> IERTAKQRLQALKANDEEAYLKLLDQAKDTRITHLLRQTDGFLKQLASSVRAQQRQAAERYGEQIDIPPDESDIDEDDEESGRKIDYYAVAHRIKEEVTEQASILVGGTLKEYQLKGLQWMLSLYNNNLNGILADEMGLGKTIQTISLITYLIEKKHQQGPYLVIVPLSTLTNWNLEFDKWAPSVAKVVYKGPPNARKMQQEKIRQGKFQVLLTTYEYIIKDRPLLSKIKWFHMIIDEGHRMKNANSKLSATIQQYYSTRFRLILTGTPLQNNLAELWAMLNFVLPNIFKSAKTFDEWFNTPFANTGGQDKMELTEEEQILVIRRLHKVLRPFLLRRLKKDVEKDLPDKTEKVIKCKFSALQARLYKQMVTHQKIAVSDA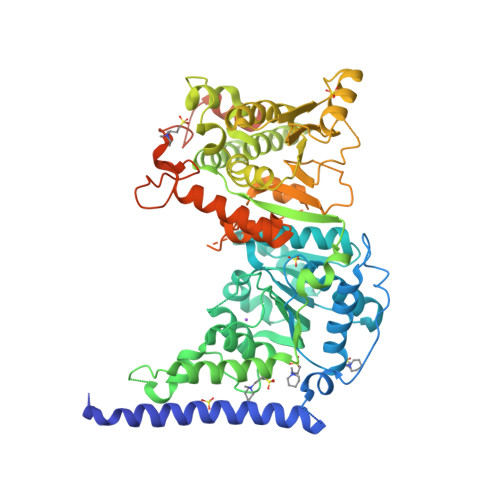NGGKTGARGLSNMIMQLRKLCNHPFVFDEVENQMNPANVSNDLLWRTAGKFELLDRILPKYKATGHRVLMFFQMTAIMDIMEDFLRFRGLHYLRLDGTTKSEDRSELLRQFNQPDSPYFMFLLSTRAGGLGLNLQTADTVIIYDSDWNPHQDLQAQDRAHRIGQKNEVRILRLISSASVEEKILERARFKLDMDGKVIQAGRFDNKSSETDRDAMLRTLLETADMAESGEQEEMDDDELNMILARNEEELAIFQKLDEERSRDPIYGTAPGCQGVPRLMTEDELPDIYLNEGNPVEEEVEMALGRGARERTKVKYDDGLTEEQWLMAVDDDEDTPEAAAARKAARREKRELN> MGSKNESTASKASGTASEKKKIEYLDKTYEVTVPTDKIAITGSVESMEDAKLLDVHPQGAISFSGKFPDMFKDITDKAEPTGEKMEPNIEKILEMKPDVILASTKFPEKTLQKISTAGTTIPVSHISSNWKENMMLLAQLTGKEKKAKKIIADYEQDLKETKTKINDKAKDSKALVIRIRQGNIYIYPEQVYFNST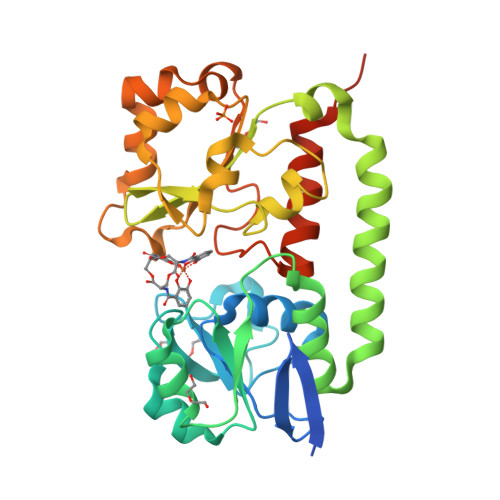LYGDLGLKAPNEVKAAKAQELISLEKLSEMNPDHIFVQFSDDENADKPDALKDLEKNPIWKSLKAVKEDHVYVNSVDPLAQGGTAWSKVRFLKAAAEKLTQNKLAAALEHHHHHH[(2R)-1-([1,2,4]triazolo[1,5-a]pyrimidin-7-yl)pyrrolidin-2-yl]methyl 2-methoxybenzoate | C18 H19 N5 O3 | 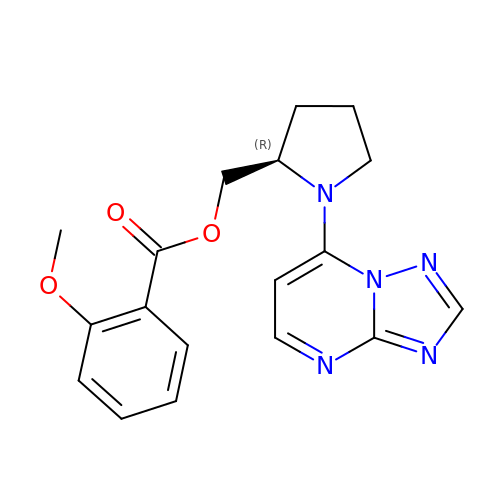QRTGQCHFTKWKOO-CYBMUJFWSA-N> MSPILAKNIVYVAQIKGQITSYTYDQFDRYITIAEQDNAEAIIIELDTPGGRADAMMNIVQRIQQSKIPVIIYVYPPGASAASAGTYIALGSHLIAMAPGTSIGACRPILGYSQNGSIIEAPPAITNYFIAYIKSLAQESGRNATIAEEFITKDLSLTPEEALKYGVIEVVARDINELLKKSNGMKTKIPVNGR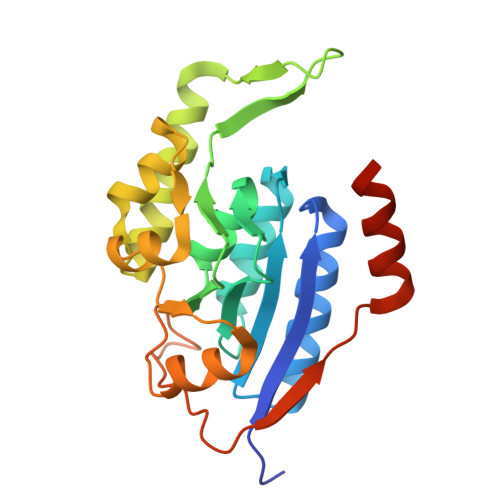YVTLNFTNVEVRYLAPSFKDKLISYITDLEHHHHHH>MLSERMLKALNDQLNRELYSAYLYFAMAAYFEDLGLEGFANWMKAQAEEEIGHALRFYNYIYDRNGRV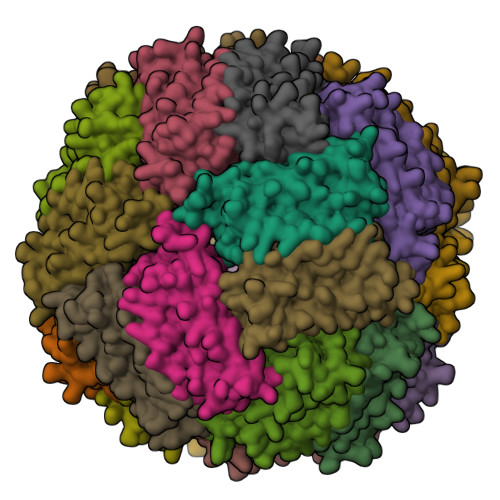ELDEIPKPPKEWESPLKAFEAAYEHEKFISKSIYELAALAEEEKDYSTRAFLEWFINEQVEEEASVKKILDKLKFAKDSPQILFMLDKELSARAPKLPGLLMQGGE[36x]HYDROGENOBYRINIC ACID | C45 H60 N4 O14 | 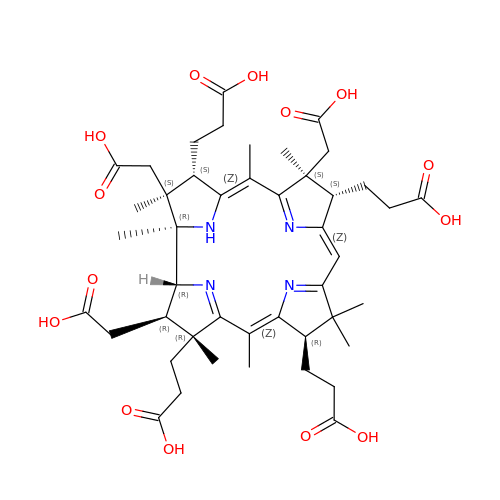MYMATQFDUQLSCD-ZPZWDRINSA-N> MPAPAASGAAAVLSKDIARSFRWMQAFAAVKGKPTAGSC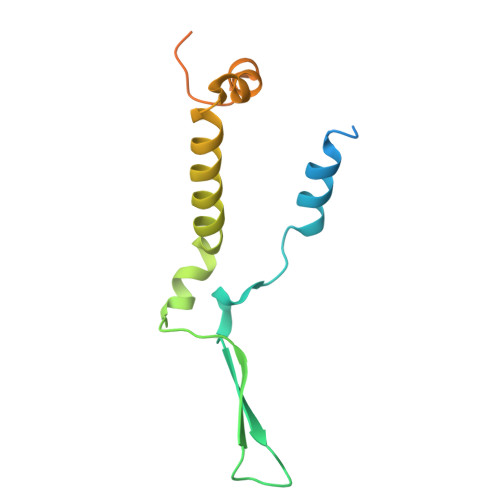AAGTAVVNPEDPTKVTLKGRYTNFSLQHIWEKYDYLQTHLLLRECMLSQVAKNPRLLDPEINAGLTPTVFMRVPPETQDPETQAKAAPQKGQAN>[4x]SASASAMLSRKGIIPEEYVLTRLAEDPAEPRYRARQRRARFVSKKGNCNVAHKNIREQGRFLQDVFTTLVDLKWPHTLLIFTMSFLCSWLLFAMAWWLIAFAHGDLAPSEGTAEPCVTSIHSFSSAFLFSIEVQVTIGFGGRMVTEECPLAILILIVQNIVGLMINAIMLGCIFMKTAQAHRRAETLIFSKHAVIALRHGRLCFMLRVGDLRKSMIISATIHMQVVRKTTSPEGEVVPLHQVDIPMENGVGGNSIFLVAPLIIYHVIDANSPLYDLAPSDLHHHQDLEIIVILEGVVETTGITTQARTSYLADEILWGQRFVPIVAEEDGRYSVDYSKFGNTIKVPTPLCTARQLDEDHSLLEALTLASARGPLRKRSVPMAKAKPKFSISPDSLSSNSLEVLFQG;>MPLAFCGSENHSAAYRVDQGVLNNGCFVDALNVVPHVFLLFITFPILFIGWGSQSSKVHIHHSTWLHFPGHNLRWILTFMLLFVLVCEIAEGILSDGVTESHHLHLYMPAGMAFMAAVTSVVYYHNIETSNFPKLLIALLVYWTLAFITKTIKFVKFLDHAIGFSQLRFCLTGLLVILYGMLLLVEVNVIRVRRYIFFKTPREVKPPEDLQDLGVRFLQPFVNLLSKGTYWWMNAFIKTAHKKPIDLRAIGKLPIAMRALTNYQRLCEAFDAQVRKDIQGTQGARAIWQALSHAFGRRLVLSSTFRILADLLGFAGPLCIFGIVDHLGKENDVFQPKTQFLGVYFVSSQEFLANAYVLAVLLFLALLLQRTFLQASYYVAIETGINLRGAIQTKIYNKIMHLSTSNLSMGEMTAGQICNLVAIDTNQLMWFFFLCPNLWAMPVQIIVGVILLYYILGVSALIGAAVIILLAPVQYFVATKLSQAQRSTLEYSNERLKQTNEMLRGIKLLKLYAWENIFRTRVETTRRKEMTSLRAFAIYTSISIFMNTAIPIAAVLITFVGHVSFFKEADFSPSVAFASLSLFHILVTPLFLLSSVVRSTVKALVSVQKLSEFLSSAEIREEQCAPHEPTPQGPASKYQAVPLRVVNRKRPAREDCRGLTGPLQSLVPSADGDADNCCVQIMGGYFTWTPDGIPTLSNITIRIPRGQLTMIVGQVGCGKSSLLLAALGEMQKVSGAVFWSSLPDSEIGEDPSPERETATDLDIRKRGPVAYASQKPWLLNATVEENIIFESPFNKQRYKMVIEACSLQPDIDILPHGDQTQIGERGINLSGGQRQRISVARALYQHANVVFLDDPFSALDIHLSDHLMQAGILELLRDDKRTVVLVTHKLQYLPHADWIIAMKDGTIQREGTLKDFQRSECQLFEHWKTLMNRQDQELEKETVTERKATEPPQGLSRAMSSRDGLLQDEEEEEEEAAESEEDDNLSSMLHQRAEIPWRACAKYLSSAGILLLSLLVFSQLLKHMVLVAIDYWLAKWTDSALTLTPAARNCSLSQECTLDQTVYAMVFTVLCSLGIVLCLVTSVTVEWTGLKVAKRLHRSLLNRIILAPMRFFETTPLGSILNRFSSDCNTIDQHIPSTLECLSRSTLLCVSALAVISYVTPVFLVALLPLAIVCYFIQKYFRVASRDLQQLDDTTQLPLLSHFAETVEGLTTIRAFRYEARFQQKLLEYTDSNNIASLFLTAANRWLEVRMEYIGACVVLIAAVTSISNSLHRELSAGLVGLGLTYALMVSNYLNWMVRNLADMELQLGAVKRIHGLLKTEAESYEGLLAPSLIPKNWPDQGKIQIQNLSVRYDSSLKPVLKHVNALIAPGQKIGICGRTGSGKSSFSLAFFRMVDTFEGHIIIDGIDIAKLPLHTLRSRLSIILQDPVLFSGTIRFNLDPERKCSDSTLWEALEIAQLKLVVKALPGGLDAIITEGGENFSQGQRQLFCLARAFVRKTSIFIMDEATASIDMATENILQKVVMTAFADRTVVTIAHRVHTILSADLVIVLKRGAILEFDKPEKLLSRKDSVFASFVRADK[4x]

A broad and rich body of literature based on decades of study describes the biochemical and functional properties of KATP channels (Aguilar-Bryan and Bryan, 1999; Aguilar-Bryan et al., 1998; Ashcroft et al., 2017; Ashcroft and Ashcroft, 1992; Hibino et al., 2010; Nichols, 2016; 2006). These channels were found to be large oligomeric complexes composed of four sulphonylurea receptor (SUR) subunits, which belong to the ABCC family of ABC transporters, and four Kir6 subunits, which are members of the inward rectifier potassium channel family. The focus of this study is the human KATP channel composed of SUR1 and Kir6.2, which are found in pancreatic beta cells where they play a major role in regulating insulin secretion. By virtue of their sensitivity to both ATP and ADP, these channels are thought to couple cellular metabolism to membrane excitability. Three naturally occurring ligands control the activity of KATP channels: PIP2 is required for activity, ATP inhibits activity, and ADP potentiates activity.

Cryo-EM reconstructions revealed two major conformations. One is similar to the published structure (‘propeller’ form) with the exception that the NBDs are closed in our structure. Upon further classification and refinement, the propeller form was determined to 5.6 Å resolution and the quatrefoil form was determined to 3.9 Å resolution. Although the final propeller form EM map is of lower resolution than that of the quatrefoil form, secondary structural elements are well defined. In addition, the L0-loop is clearly visible in the propeller form albeit at lower resolution. In the propeller form the ATP-binding site on Kir6.2 is buttressed by the lasso extension, which attaches SUR1 to the CTD. In the propeller form, in which the lasso extension/Kir6 interface is intact, the SUR1 transporter modules are held with an offset with respect to the hydrophobic membrane plane, as defined by the position of the Kir6.2 channel and TMD0 domains. The consequence of holding the transport modules at a shifted position with respect to the pore in the propeller form should be strain exerted on the lasso extension/Kir6 interface in the propeller form. When we compare the NBD-dimerized propeller form in this study with the published NBD-open propeller form, we observe that dimerization causes a slight tilting of NBD1 away from the center of the complex. Thus, dimerization appears to exert force on the lasso extension away from the channel.> GSMSEQSICQARAAVMVYDDA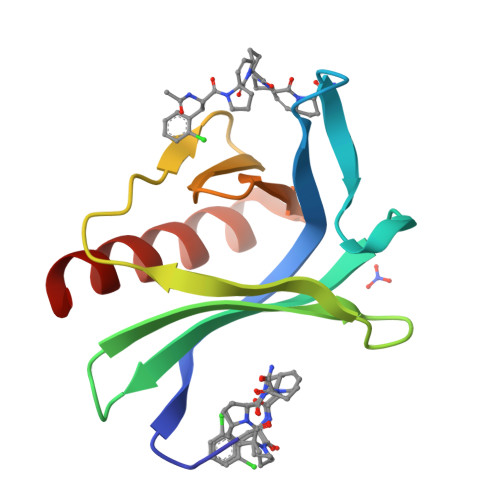NKKWVPAGGSTGFSRVHIYHHTGNNTFRVVGRKIQDHQVVINCAIPKGLKYNQATQTFHQWRDARQVYGLNFGSKEDANVFASAMMHALEVL> METAIWIKNSKLPAVLVAAGAFDAAVQALSKQVGVVKLEPLKKYFTNIYEGCRTYIPSTPCELPAQLGYVRAYDDTVSEDQILPYVPGLDVVNEKMNEGYKNFKLNKPDIAIECFREAIYRITLLMVDDAEDEKLAHKILETAREYILGLSIELERRSLKEGNTVRMLELAAYFTKAKLSPIHRTNALQVAMSQHFKHKNFLQASYFAGEFLKIISSGPRAEQARKIKNKADSMASDAIPIDFDPYAKFDICAATYKPIYEDTPSVSDPLTGSKYVITEKDKIDRIAMISKIGAPASGLRIRV;> MGSSHHHHHHSQDPMDYFNIKQNYYTGNFVQCLQEIEKFSKVTDNTLLFYKAKTL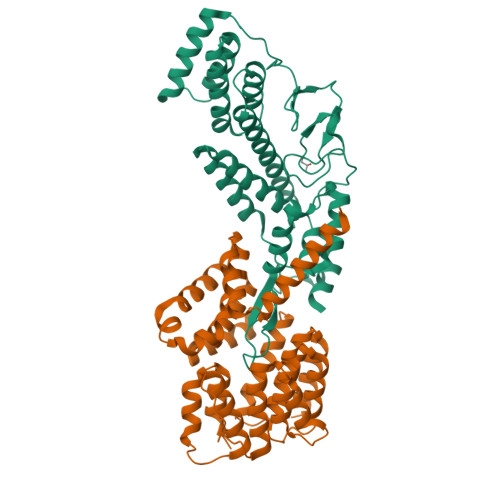LALGQYQSQDPTSKLGKVLDLYVQFLDTKNIEELENLLKDKQNSPYELYLLATAQAILGDLDKSLETCVEGIDNDEAEGTTELLLLAIEVALLNNNVSTASTIFDNYTNAIEDTVSGDNEMILNLAESYIKFATNKETATSNFYYYEELSQTFPTWKTQLGLLNLHLQQRNIAEAQGIVELLLSDYYSVEQKENAVLYKPTFLANQITLALMQGLDTEDLTNQLVKLDHEHAFIKHHQEIDAKFDELVRKYDTSN> GKNVMVEPHRHEGVFICRGKEDALVTKNLVPGE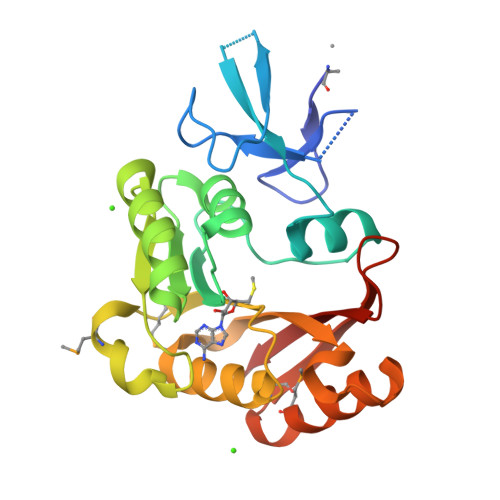SVYGEKRVSISEGDDKIEYRAWNPFRSKLAAAILGGVDQIHIKPGAKVLYLGAASGTTVSHVSDIVGPDGLVYAVEFSHRSGRDLINLAKKRTNIIPVIEDARHPHKYRMLIAMVDVIFADVAQPDQTRIVALNAHTFLRNGGHFVISIKANCIDSTASAEAVFASEVKKMQQENMKPQEQLTLEPYERDHAVVVGVYRP> MEEDIACVKDLVSKYLANNERLSRQKLAFLVQTEPRMLLMEGLKLLSLCIEVDSCNANGCEHNSEDKSVERILHDHGVLTPSLCFVVPDGYKLTGNVLILLECFVRSSPANFEQKYVEDFKKLEQLKEDLKSVDINLIPLIDGRTSFYNEQIPDWVNDKLRDTLFSLLKYAQESNSLFEESEYSRLCESLSMTSGRLSGVESLNALLDNRSNHYEEVIASCHQGINNKLTAHEVKLQIEEEYQVFRNRLRKGEIEGQFLKVEKNQLLNEFNNL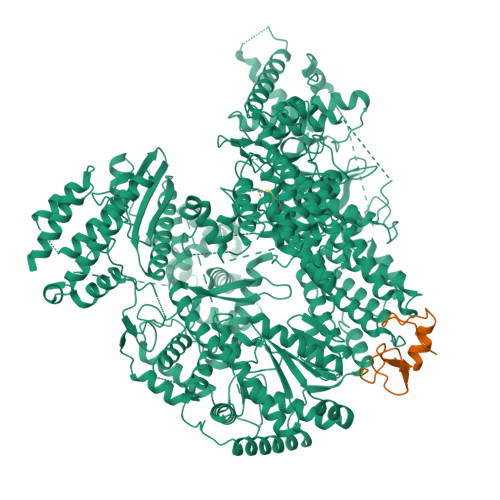YADKVAEKDSVEHLTHQFKRASPILRFLYANISKGDNGEGNLIIGECQMQCWRSFLNKVKSMRILNTRRKLLLIFDALILLASKHDQVRKKPLRGWLGTCFVSVNDRLVSLESTKKDLKKWVERRQQVERSRTMQSFQCPSKNQILNSIFQKTISKATTALRDVGISVDHYKIDMEVICPDGYDLIMDFDVSGVTPTISYQRSEEEAFPYIMGDVDLLKTTDLERLSSLSLALVNSMKTSSTVKLRQNEFGPARYQVVKCKEAYCQEFSLGETEFQLIYQKTGECSKCYAINDNRVGEVCSFYADPKRYFPAIFSAEVLQTTVSTMISWIEDCNELEEQLDKIRSLTKMILILILAHPSKRSQKLLQNLRYFIMAYVSDYYHKDLIDKVREELITDVEFLLYRLLRTLMGLVLSEDVKSMMTNRFKFILNISYMCHFITKETPDRLTDQIKCFEKFLEPKVKFGHVSINPADTATEEELDDMVYNAKKFLSKGGCTSAKGPSYKKPGVSKKYLSLLTSSFNNGSLFKEREVKKEIKDPLITSGCATALDLASNKSVVVNKYTDGSRVLNYDFNKLTALAVSQLTEVFSRKGKHLLNKQDYEYKVQQAMSNLVLGSKQHKGDADEADLDEILLDGGASTYFNQLKETVEKIVDQYREPVKMGSGSNDGDQPSINDLDEIVSNKFYIRLIKGELSNHMVEDFDHDVLPDKFYEEFCDAVYENSKLKEKYFYCGHMSQCPIGELTKAVSTRTYLDHEYFQCFKSILLIMNANALMGKYTHYKSRNLNFKFDMGKLSDDARISERESNSEALSKALSLTNCTTAMLKNLCFYSQESPQSYNSVGPDTGRLKFSLSYKEQVGGNRELYIGDLRTKMFTRLIEDYFEALSSQLSGSCLNNEKEFENAILSMKLNVSMAHVSYSMDHSKWGPMMCPFLFLTVLQNLIFLSKDLQADIKGRDYLSTLLMWHMHKMVEIPFNVVSAMMKSFIKAQLGLRKKTKQSITEDFFYSNFQIGVVPSHISSILDMGQGILHNTSDFYALITERFINYAISCVCGGTIDAYTSSDDQISLFDQTLTELLHRDPEEFRALMEFHYYMSDQLNKFVSPKSVIGRFVAEFKSRFFVWGDEVPLLTKFVAAALHNIKCKEPHQLAETIDTIVDQSVANGVPVHLCNLIQIRTLSLLQYARYPIDPFLLNCETDVRDWVDGNRSYRIMRQIEGLIPDACSKIRSMLRRLYNRLKTGQLHEEFTTNYLSSEHLSSLKNLCELLGVEPPSESDLEYSWLNLAAHHPLRMVLRQKIIYSGAVNLDDEKIPTIVKTIQNKLSSTFTRGAQKLLSEAINKSAFQSSIASGFVGLCRTLGSKCVRGPNKENLYIKSIQSLITGTQGIELLTNSIGVQYWRVPLGLRNKSESVVSYFRPLLWDYMCISLSTAIELGAWVLGDPKTTKALDFFKHNPCDYFPLKPTASKLLEDRVGLNHIIHSLRRLYPSVFEKHILPFMSDLASTKMKWSPRIKFLDLCVALDVNCEALSLVSHIVKWKREEHYIVLSSELRFSHTRTHEPMVEERVVSTSDAVDNFMRQIYFESYVRPFVATTRTLGSFTWFPHRTSIPEGEGLHRLGPFSSFVEKVIHKGVERPMFKHDLMMGYAWIDFDIEPARFNQNQLIASGLVDSKFDSLEDFFDAVASLPTGSAKLSQTVRFRIKSQDASFRESFAIHLDYIGSMNQQAKYLVHDVTAMYSGAVSPCVLSDCWRLVLSGPTFKGKPVWYVDTEVINEFLVDTNQLGHVTPVEVVVDMEKLQFAEYDFMLVGPCAEPVPLVVRRGGLWECEKKLASFTPVIQDQDLEMFVREVGDTSSDLLIRALSDMITDRLGLRMQWSGVDIVSTLRAAAPGNAEVLSAVLEVVDNWVEFKGYALCYSKSRGRVMVQSSSGKLRLKGRTCEELTEGGEHVEDIE;> MGNKQVKAPEARNSPRASLIPDATHLGPQFCKSCWFENKGLVECNNHYLCLNCLTLLLGVSSRCPICKMPLPTRLRPSAAPTAPPAEAGDNTRPPPYSP> MADFARSLSITTPEEMIEKAKGETAYLPCKFTLSPEDQGPLDIEWLISPADNQKVDQVIILYSGDKIYDDYY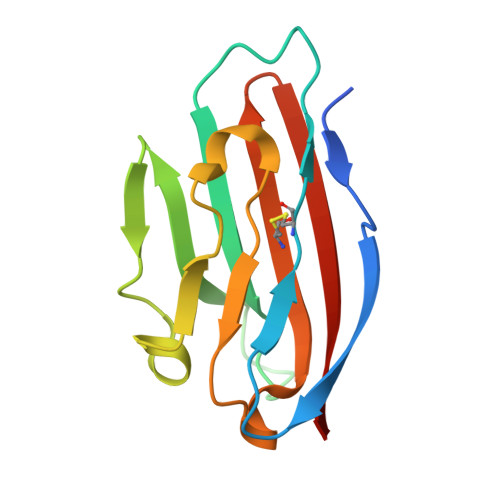PDLKGRVHFTSNDLKSGDASINVTNLQLSDIGTYQCKVKKAPGVANKKIHLVVLGK>[2x]MLPQRLHPSRLLALALFSLVLGLAGCQTKPPQTGLSAEQIAV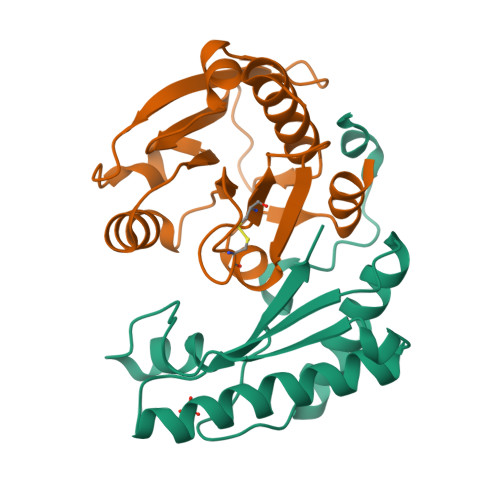PQEQGFELRDEGWEFGMSSKVLFGNNLDRLNPDSRNTLTKIARALLAVDIDKVRLEGHTDNYGDEGYNQKLSERRAESVAAVFREAGMPAANIEVRGLGMSKPVADNKTRAGRSENRRVAIIVPAE;>MPSLPTLQPLDLYRRTLACLVLAVSCLGGGGLWADDARTSIEQRSNAVSQVLLGIFSYVRWPKEPAVLQLCVVGPTEYADGLLRGMVQANGRRVHAERRAVDNPDLGTLCNVIYLGVVDERERQQVFRSLAGHPVLSISERGTECSVGSMFCLNVGGPRITFEANLDSIARSGVRVHPSVLKLARRQATP[2x]> GELPEKSKLQEIYQELT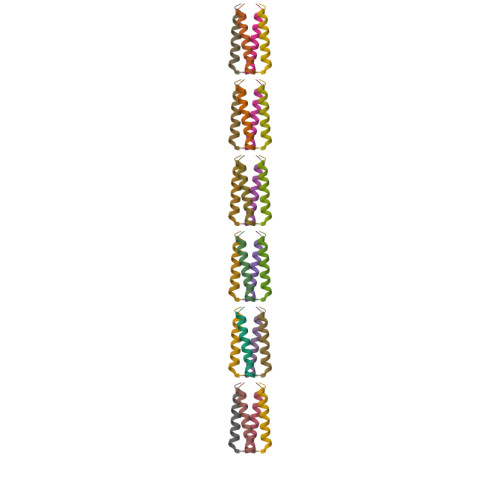RLKAAVGELPEKSKLQEIYQELTRLKAAVGELPEKSKLQEIYQELTRLKAAVGELPEKSKLQEIYQELTRLKAAVGELPEKSKLQEIYQELTELKAAVGELPEKSKLQEIYQELTQLKAAVGELPDQSKQQQIYQELTDLKTAFERLGHH> AMDLRVGRKFRIGRKIGSGSFGDIYHGTNLISGEEVAIRLESIRSRHPQLDYESRVYRYLSGGVGIPFIRWFGREGEYNAMVIDLLGPSLEDLFNYCHRRFSFKTVIMLALQMFCRIQYIHGRSFIHRDIKPDNFLMGVGRRGSTVHVIDFGLS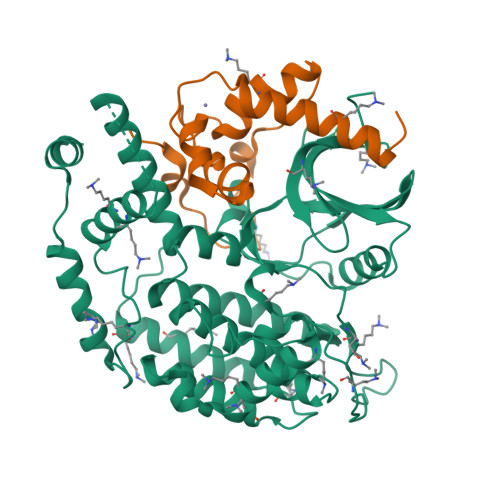KKYRDFNTHRHIPYRENKSLTGTARYASVNTHLGIEQSRRDDLESLGYVLIYFCKGSLPWQGLKATTKKQKYDRIMEKKLNVSVETLCSGLPLEFQEYMAYCKNLKFDEKPDYLFLARLFKDLSIKLEYHNDHLFDWTMLRYTKAMVEKQRDLLIEKGDLNANSNAASASNSTDNKSETFNKIKLLAMKKFPTHFHYYKNEDKHNPSPEEIKQQTILNNNAASSLPEELLNALDKGMENLR;> EATECLTRSNLKKLQEKIFDRELNDIACDHCLCSTENRRDIKYSRLWFLFELEMSENWNENLRLSCYNKYVYSAIDESWKMENILLKEQEKHYEYFPIGQLLIPN>HHHHHHMATETNYPVPYR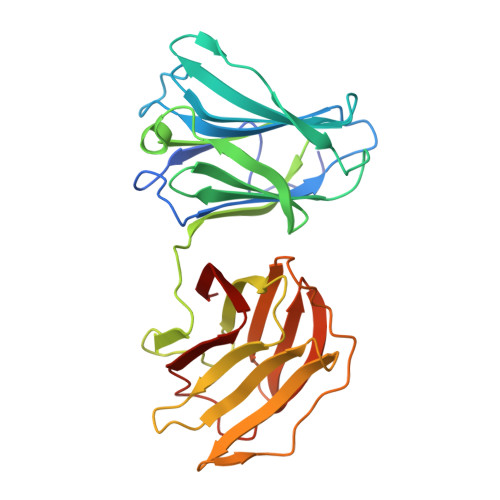SKLTEPFEPGQTLIIKGKTAEDSVRFTINLHNTSADFSGNDVPLHISVRFDEGKIVFNTFSKGEWGKEERKSNPYKKGDDIDIRIRAHDSKFSISVDQKEVKEYEHRVPLSSVTHFSVDGDILITYIHWGGKYYPVPYESGLAGDGLAPGKSLLIFATPEKKGKRFHINLLKKNGDIALHFNPRFDEKAIVRNSLISGEWGNEEREGKNPLEKGIGCDLEFRNEEYAFQIYVDGERFATYAHRLDPHDINGLQIGGDVEVTGIQMV[2x]> MRSWLGEGVRAQQWLSVCAGRQDMVLATVLLIAIVMMLLPLPTWMVDILITINLMFSVILLLIAIYLSDPLDLSVFPSLLLITTLYRLSLTISTSRLVLLQHNAGNIVDAFGKFVVGGNLTVGLVVFTIITIVQFIVITKGIERVAEVSARFSLDGMPGKQMSIDGDLRAGVIDADHAR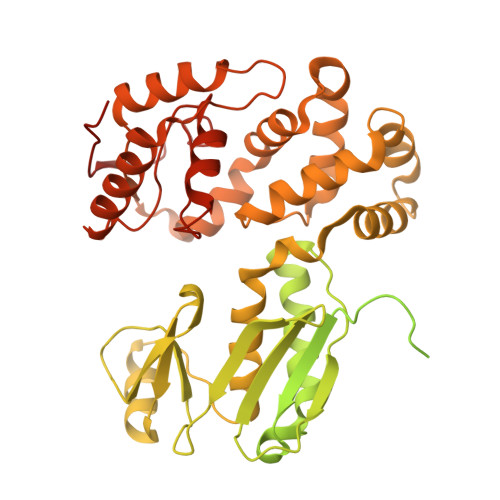TLRQHVQQESRFLGAMDGAMKFVKGDTIAGIIVVLVNIIGGIIIAIVQYDMSMSEAVHTYSVLSIGDGLCGQIPSLLISLSAGIIVTRVPGEKRQNLATELSSQIARQPQSLILTAVVLMLLALIPGFPFITLAFFSALLALPIILIRRKKSVVSANGVEAPEKDSMVPGACPLILRLSPTLHSADLIRDIDAMRWFLFEDTGVPLPEVNIEVLPEPTEKLTVLLYQEPVFSLSIPAQADYLLIGADASVVGDSQTLPNGMGQICWLTKDMAHKAQGFGLDVFAGSQRISALLKCVLLRHMGEFIGVQETRYLMNAMEKNYSELVKELQRQLPINKIAETLQRLVSERVSIRDLRLIFGTLIDWAPREKDVLMLTEYVRIALRRHILRRLNPEGKPLPILRIGEGIENLVRESIRQTAMGTYTALSSRHKTQILQLIEQALKQSAKLFIVTSVDTRRFLRKITEATLFDVPILSWQELGEESLIQVVESIDLSEEELADNEEHHHHHH> MSVEKIPGYTYGETENRAPFNLEDLKLLKEAVMFTAEDEEYIQKAGEVLEDQVEEILDTWYGFVGSHPHLLYYFTSPDGTPNEKYLAAVRKRFSRWILDTSNRSYDQAWLDYQYEIGLRHHRTKKNQTDN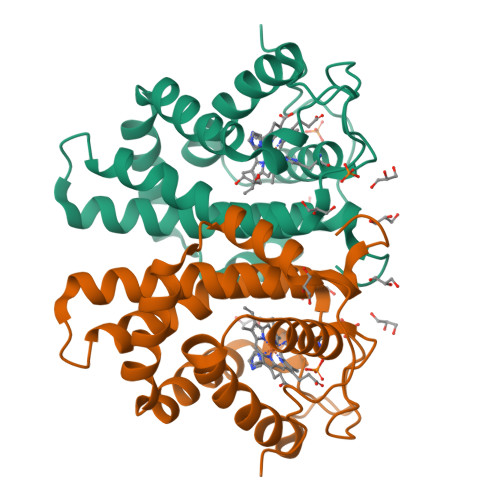VESVPNIGYRYLVAFIYPITATMKPFLARKGHTPEEVEKMYQAWFKATTLQVALWSYPYVKYGDF Gcn5 is a member of the GNAT (Gcn5-related N-acetyltransferase) family of histone acetyltransferases that acetylate the N-terminal tails of histones H3 and H2B at the promoters of inducible genes and are broadly implicated in transcriptional regulation. The active site of Gcn5 contains two grooves where acetyl-CoA and peptide bind, which intersect near the β-mercaptoethylamine moiety of coenzyme A and the target lysine. The ternary complex between Gcn5, acetyl-CoA and peptide forms through a fully ordered mechanism, as binding to acetyl-CoA brings about a structural rearrangement that widens the peptide-binding groove within the Gcn5 active site. Whereas Gcn5L2 robustly catalyzes lysine acetylation, the acyltransferase activity of Gcn5L2 becomes progressively weaker with increasing acyl-chain length.

To elucidate the structural basis for the ability of Gcn5L2 to discriminate among different acyl-CoA cofactors, we determined the structures of human Gcn5L2 bound to propionyl-CoA and butyryl-CoA to 2.0 and 2.1 Å resolution, respectively. Compared with the structure of human Gcn5L2 bound to acetyl-CoA, the structures reported here are very similar; the root-mean-square difference (r.m.s.d.) in Cα positions is 0.13 Å for the structure of human Gcn5L2 in complex with propionyl-CoA and 0.24 Å for its structure in complex with butyryl-CoA. To determine whether human Gcn5 can similarly use other acyl-CoAs as a cofactor, we measured Gcn5 activity in the presence of either propionyl-CoA or butyryl-CoA and histone H3 peptide. We found that human Gcn5L2 efficiently acetylates and propionylates peptides, while its butyrylating activity is nearly undetectable. Based on these relative rate measurements, Gcn5L2 is unlikely to contribute significantly to lysine butyrylation in vivo but may be capable of catalyzing lysine propionylation under physiological conditions. We have determined crystal structures that describe how Gcn5 accommodates propionyl-CoA in its active site and provide a structural mechanism that explains our biochemical data showing that human Gcn5 discriminates between different acyl-CoA molecules. To understand how Gcn5 discriminates between the different acyl-chain donors, we determined structures of the catalytic domain of human Gcn5L2 in complex with propionyl-CoA and butyryl-CoA to 2.0 and 2.1 Å resolution, respectively. These structures reveal that the active site of Gcn5 can accommodate longer acyl chains without major structural rearrangements, but that the butyryl chain would sterically clash with an incoming lysine residue.

> GSGIIEFHVIGNSLTPKANRRVLLWLVGLQNVFSHQLPRMPKEYIARLVFDPKHKTLALIKDGRVIGGICFRMFPTQGFTEIVFCAVTSNEQVKGYGTHLMNHLKEYHIKHNILYFLTYADEYAIGYFKKQGFSKDIKVPKSRYLGYIKDYEGATLMECELNPRIPYT> MPNPPSFKSHKQNLFNSNNNQHANSVDSFDLHLDDSFDAALDSLQINNNPEPLSKHNTVGDRESFEMRTVDDLDNFSNHSSDSHRKSSNTDTHPLMYDNRLSQDDNFKFTNIASSPPSSSNNIFSKALSYLKVSNTKNWSKFGSPIELSDQHIEREIHPDTTPVYDRNRYVSNELSNAKYNAVTFVPTLLYEQFKFFYNLYFLVVALSQAVPALRIGYLSSYIVPLAFVLTVTMAKEAIDDIQRRRRDRESNNELYHVITRNRSIPSKDLKVGDLIKVHKGDRIPADLVLLQSSEPSGESFIKTDQLDGETDWKLRVACPLTQNLSENDLINRISITASAPEKSIHKFLGKVTYKDSTSNPLSVDNTLWANTVLASSGFCIACVVYTGRDTRQAMNTTTAKVKTGLLELEINSISKILCACVFALSILLVAFAGFHNDDWYIDILRYLILFSTIIPVSLRVNLDLAKSVYAHQIEHDKTIPETIVRTSTIPEDLGRIEYLLSDKTGTLTQNDMQLKKIHLGTVSYTSETLDIVSDYVQSLVSSKNDSLNNSKVALSTTRKDMSFRVRDMILTLAICHNVTPTFEDDELTYQAASPDEIAIVKFTESVGLSLFKRDRHSISLLHEHSGKTLNYEILQVFPFNSDSKRMGIIVRDEQLDEYWFMQKGADTVMSKIVESNDWLEEETGNMAREGLRTLVIGRKKLNKKIYEQFQKEYNDASLSMLNRDQQMSQVITKYLEHDLELLGLTGVEDKLQKDVKSSIELLRNAGIKIWMLTGDKVETARCVSISAKLISRGQYVHTITKVTRPEGAFNQLEYLKINRNACLLIDGESLGMFLKHYEQEFFDVVVHLPTVIACRCTPQQKADVALVIRKMTGKRVCCIGDGGNDVSMIQCADVGVGIVGKEGKQASLAADFSITQFCHLTELLLWHGRNSYKR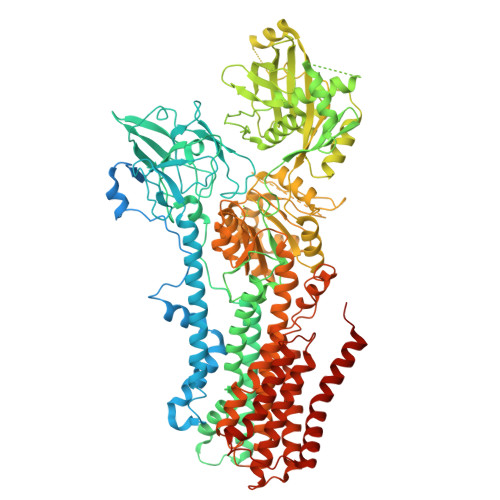SAKLAQFVMHRGLIIAICQAVYSICSLFEPIALYQGWLMVGYATCYTMAPVFSLTLDHDIEESLTKIYPELYKELTEGKSLSYKTFFVWVLLSLFQGSVIQLFSQAFTSLLDTDFTRMVAISFTALVVNELIMVALEIYTWNKTMLVTEIATLLFYIVSVPFLGDYFDLGYMTTVNYYAGLLVILLISIFPVWTAKAIYRRLHPPSYAKVQEFATP N-(2,3-dihydro-1,4-benzodioxin-6-yl)-2-(8-methyl[1]benzopyrano[4,3-c]pyrazol-1(4H)-yl)acetamide 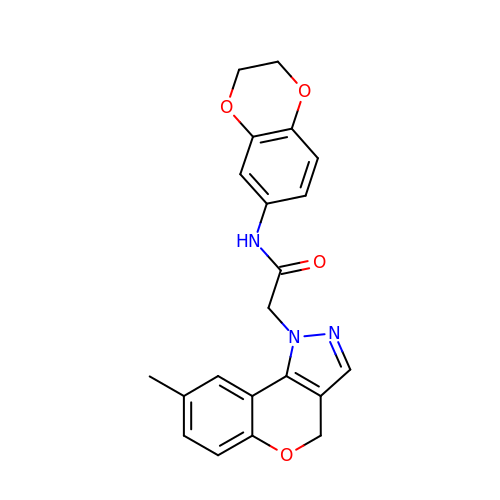| C21 H19 N3 O4 | YHHIKABCYPQVLY-UHFFFAOYSA-N>MPFPFGKSHKSPADIVKNLKESMAVLEKQDISDKKAEKATEEVSKNLVAMKEILYGTNEKEPQTEAVAQLAQELYNSGLLSTLVADLQLIDFEGKKDVAQIFNNILRRQIGTRTPTVEYICTQQNILFMLLKGYESPEIALNCGIMLRECIRHEPLAKIILWSEQFYDFFRYVEMSTFDIASDAFATFKDLLTRHKLLSAEFLEQHYDRFFSEYEKLLHSENYVTKRQSLKLLGELLLDRHNFTIMTKYISKPENLKLMMNLLRDKSRNIQFEAFHVFKVFVANPNKTQPILDILLKNQAKLIEFLSKFQNDRTEDEQFNDEKTYLVKQIRDLKRPAQQEA[2x];>MSSFLPEGGCYELLTVIGKGFEDLMTVNLARY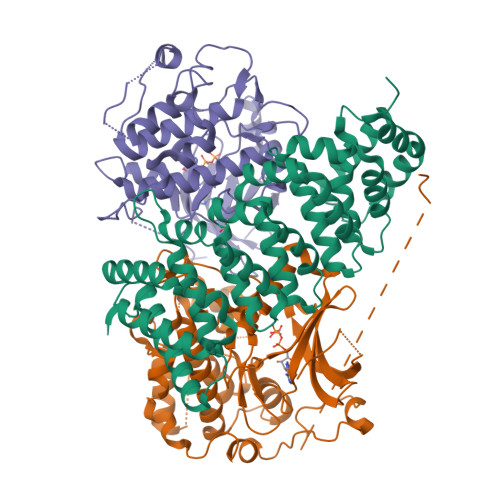KPTGEYVTVRRINLEACSNEMVTFLQGELHVSKLFNHPNIVPYRATFIADNELWVVTSFMAYGSAKDLICTHFMDGMNELAIAYILQGVLKALDYIHHMGYVHRSVKASHILISVDGKVYLSGLRSNLSMISHGQRQRVVHDFPKYSVKVLPWLSPEVLQQNLQGYDAKSDIYSVGITACELANGHVPFKDMPATQMLLEKLNGTVPCLLDTSTIPAEELTMSPSRSVANSGLSDSLTTSTPRPSNGDSPSHPYHRTFSPHFHHFVEQCLQRNPDARPSASTLLNHSFFKQIKRRASEALPELLRPVTPITNFEGSQSQDHSGIFGLVTNLEELEVDDWEF[2x];>AKLIGKYLMGDLLGEGSYGKVKEVLDSETLCRRAVKILKKKKLRRIPNGEANVKKEIQLLRRLRHKNVIQLVDVLYNEEKQKMYMVMEYCVCGMQEMLDSVPEKRFPVCQAHGYFCQLIDGLEYLHSQGIVHKDIKPGNLLLTTGGTLKISALGVAEALHPFAADDTCRTSQGSPAFQPPEIANGLDTFSGFKVDIWSAGVTLYNITTGLYPFEGDNIYKLFENIGKGSYAIPGDCGPPLSDLLKGMLEYEPAKRFSIRQIRQHSWFRKKHPPAEAPVPIPPSPDTKDRWRSMTVVPYLEDLHGA[2x]> LKFSPQLLSLLSLKTSLSGPPSAFQDWKVPVNGQNDAVWCSWSGVVCDNVTAQVISLDLSHRNLSGRIPIQIRYLSSLLYLNLSGN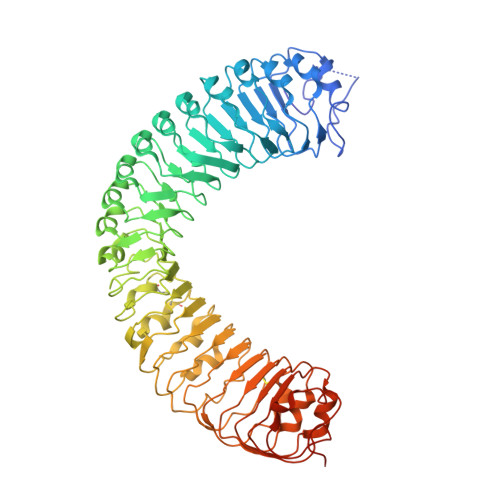SLEGSFPTSIFDLTKLTTLDISRNSFDSSFPPGISKLKFLKVFNAFSNNFEGLLPSDVSRLRFLEELNFGGSYFEGEIPAAYGGLQRLKFIHLAGNVLGGKLPPRLGLLTELQHMEIGYNHFNGNIPSEFALLSNLKYFDVSNCSLSGSLPQELGNLSNLETLFLFQNGFTGEIPESYSNLKSLKLLDFSSNQLSGSIPSGFSTLKNLTWLSLISNNLSGEVPEGIGELPELTTLFLWNNNFTGVLPHKLGSNGKLETMDVSNNSFTGTIPSSLCHGNKLYKLILFSNMFEGELPKSLTRCESLWRFRSQNNRLNGTIPIGFGSLRNLTFVDLSNNRFTDQIPADFATAPVLQYLNLSTNFFHRKLPENIWKAPNLQIFSASFSNLIGEIPNYVGCKSFYRIELQGNSLNGTIPWDIGHCEKLLCLNLSQNHLNGIIPWEISTLPSIADVDLSHNLLTGTIPSDFGSSKTITTFNVSYNQLIGPIPSGSFAHLNPSFFSSNEGLCGDLVGKPCNSDRFNAGNADIDG> MSVSGVFSKGRGIGHEATTSILRYIPRARVPWQPSRFGRENLTAADMARLWSRGRYRDGPGNYNSGYCTERTHVLEENTVSIIPRRELEKYMPDITIGPKALVTPVSLMNARNGHRVTHDLL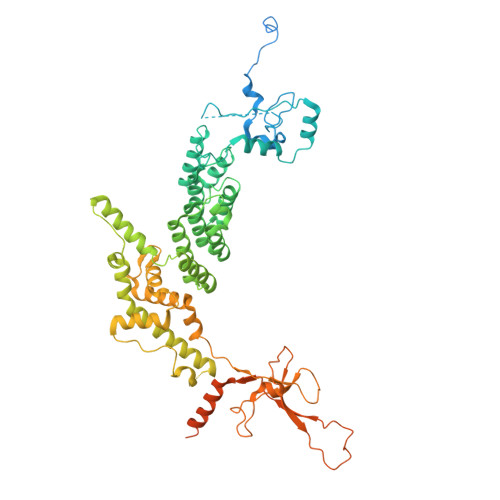HSYDPHIGRLGKPAVVDHDNITVEDPNRVGLNAATLDCRGRIYRWLRRGPFFQVDNYFRRSVKLNRDGTLPTDFVHEAPLMRKIIRLAHRGHLKAACEEYRRVTTVPPVEVYRALTACCVPGAKLADAVSIFEDGDSKLFYVSRDGEVLHNLMRCAIAARHRARIMWVYNVMRGRFYENVVVRAEVDLIWRYRIAMIALEYLLDHECAEEAAAIYSYLVEEELLRCDVHVRVGLHMREAIAAGKPITLNNDVMNATSLVRDATAVAPEVARELQRRHAQTLQNNAVEAVGAENVREGSAPWSILGPLTAIGPTAEDTMVWLQQHYGDVDVMSIMRWARFRKGKDLMAKDRPQYLARAAAWIELLSKRNREMEEVPLTYMRKSKPLVLDTNSNVRVAWQTPLMRSGGPPRLLAREEGYVFHHSNSSRFVEETYRHPGESLQSRYLALQPLHTEVSAKEDFQRLYYQAQKHHKQQERLLPVSTAAIPSRIVHHSVMSALHGVSGKGEPANRSLFTGNKSNDSHSNTGVASGTSACTDGAGSATPEF> 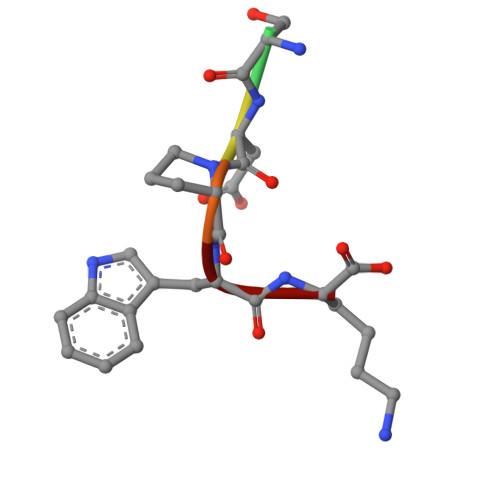GSDPWK Pif1 is a multifunctional helicase and DNA processing enzyme that has roles in genome stability. Pif1 proteins are monomeric enzymes and members of helicase superfamily 1 (SF1), while the 5′–3′ polarity of unwinding place them in the SF1B subgroup. The hPIF1 helicase has the domain architecture characteristic of the SF1B RecD2 helicase subgroup. The overall organization of these domains is similar in all nucleotide bound and free structures determined. hPIF1 has three structural domains, two RecA-like domains 1A (residues 206–381, blue in Figure 1) and 2A (residues 382–435) and domain 2B (residues 436–548, green in Figure 1) with a SRC Homology 3 (SH3)-like fold, in addition to the small functional domain 1B within domain 1A (residues 280–300, cyan in Figure 1).

The structures we report are of constructs from residues 206–641 (apo hPIF1) or 206–620 (the structures with nucleotide analogues bound). During ATP binding, represented by the AMP-PNP structure, R381 recognizes the γ-phosphate of ATP. R584 also shifts in position to interact with the ATP γ-phosphate, fixing the α13 helix (domain 2A) relative to the ATP-binding pocket, while Q346 from motif III coordinates the ATP γ-phosphate. Importantly, this conformational rearrangement of the 1A–2A inter-domain linker (W380 and R381) during nucleotide binding causes a significant ∼4 Å shift of the N-terminal end of the α9 helix, which in turn induces a structural rearrangement of the 2B domain. ATP binding results in a 4 Å movement of the N-terminus of helix α9 (helix α9 corresponds to the conserved motif A) while the C-terminus remains relatively fixed to α13, which is immobilized by interactions (R584) with the bound nucleotide.

>[2x]SRMQLSEEQAAVLRAVLKGQSIFFTGSAGTGKSYLLKRILGSLPPTGTVATASTGVAACHIGGTTLHAFAGIGSGQAPLAQCVALAQRPGVRQGWLNCQRLVIDEISMVEADLFDKLEAVARAVRQQNKPFGGIQLIICGDFLQLPPVTKGSQPPRFCFQSKSWKRCVPVTLELTKVWRQADQTFISLLQAVRLGRCSDEVTRQLQATASHKVGRDGIVATRLCTHQDDVALTNERRLQELPGKVHRFEAMDSNPELASTLDAQCPVSQLLQLKLGAQVMLVKNLSVSRGLVNGARGVVVGFEAEGRGLPQVRFLCGVTEVIHADRWTVQATGGQLLSRQQLPLQLAWAMSIHKSQGMTLDCVEISLGRVFASGQAYVALSRARSLQGLRVLDFDPMAVRCDPRVLHFYATLRRGRSL> LEMRIGHGFDVHAFGGEGPIIIGGVRIPYEKGLLAHSDGDVALHALTDALLGAAALGDIGKLFPDTDPAFKGADSRELLREAWRRIQAKG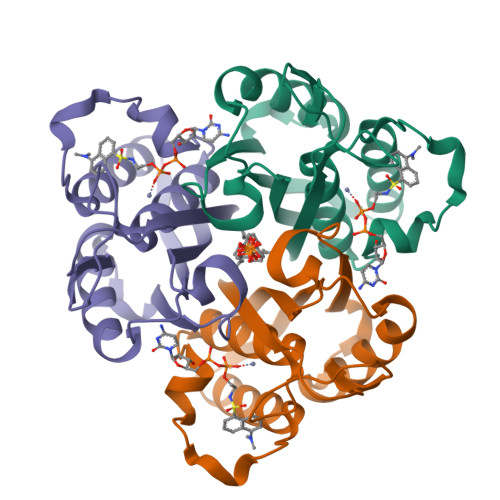YTLGNVDVTIIAQAPKMLPHIPQMRVFIAEDLGCHMDDVNVKATTTEKLGFTGRGEGIACEAVALLIKA> QNEPRIVTSEEVIIRDSLLPVTLQCNLTSSSHTLMYSYWTKNGVELTATRKNASNMEYRINKPRAEDSGEYHCVYHFVSAPKANATIEVKAA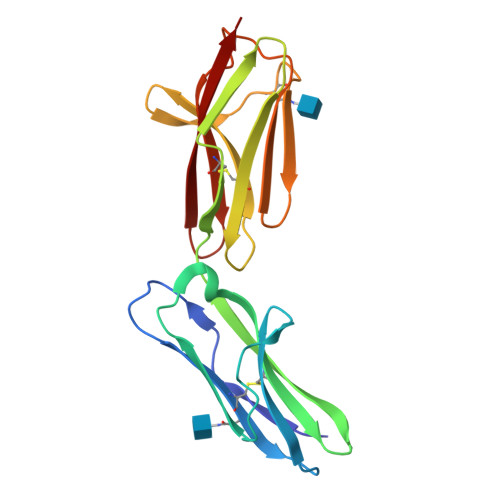PDITGHKRSENKNEGQDAMMYCKSVGYPHPEWMWRKKENGVFEEISNSSGRFFIINKENYTELNIVNLQITEDPGEYECNATNSIGSASVSTVLRVRV Dimethylsulfoxonium propionate (DMSOP) is a recently identified and abundant marine organosulfur compound with roles in oxidative stress protection, global carbon and sulfur cycling and, as shown here, potentially in osmotolerance. Microbial DMSOP cleavage yields dimethyl sulfoxide, a ubiquitous marine metabolite, and acrylate, but the enzymes responsible, and their environmental importance, were unknown. Here we report DMSOP cleavage mechanisms in diverse heterotrophic bacteria, fungi and phototrophic algae not previously known to have this activity, and highlight the unappreciated importance of this process in marine sediment environments. These diverse organisms, including Roseobacter, SAR11 bacteria and Emiliania huxleyi, utilized their dimethylsulfoniopropionate lyase ‘Ddd’ or ‘Alma’ enzymes to cleave DMSOP via similar catalytic mechanisms to those for dimethylsulfoniopropionate. Like dddY, cloned dddL, dddQ, dddW, dddK and dddU conferred DMSOP lyase activity even with equimolar DMSP present, which was not surprising considering the similar structures of DMSP and DMSOP, and that these DMSP lyases have cupin domains and similar catalytic mechanisms.

Cloned dddY from A. faecalis and Acinetobacter bereziniae conferred DMSOP lyase activity to E. coli (424.2 ± 20.6 and 359.4 ± 18.0 pmol DMSO per mg protein per minute, respectively) and purified DddY proteins yielded DMSO and acrylate from DMSOP. In contrast, DddY, DddX, DddP, DddL and Alma were more efficient (3–13.3-fold) using DMSP than DMSOP, whereas DddK, DddQ and DddU were more efficient (2–83.4-fold) with DMSOP. Note, DddP, DddX, DddY and Alma proteins generated 1.4–5-fold more DMS than DMSO when incubated with equimolar DMSP and DMSOP levels, consistent with them having significant DMSOP lyase activity but preferring DMSP as a substrate. We also solved the crystal structure of the DddY–DMSOP complex and docked DMSOP into DddQ and DddP structures.

>[2x]MHKRFLGTIFGATLTCFQAQAAQFQCQDDVKPTSYTTEEQKLVDQFWNESLIYLDQYLKALETPTGQCKDSAQATIQTYNSETGKMQTQCIMKYRDVELVAKHLKAVLAEPDKAKACFDPQKNYKAFPLYTPSAHVQNLSATSKWINRPLLTDYYKKIGGEIGAAGLELNENFLEITSRTDTTLHWTKDVSIKGLPTLWSSVGWIPFYAENPNAGSDRFRGGYLYAEVMGPWGNLRIKEIDGEKVGAEIGMTAQLFNTSAPYHYHHPQEIYMTLTKPQCIDQNKHMVMHWDNNQFKQKRSDNGWTVNIDGSKGKWKKWFSNQDPEQNWLTYFERNAIHAFHTLEGCNQTIKNSGLVTVWARTTAQDNNQTTQLCRPMTGAKDIKTMKPEDKAICDLDDWKPHHHHHH(5S)-3-(3,6-dihydro-2H-pyran-4-yl)-7-[5-(prop-1-yn-1-yl)pyridin-3-yl]-5'H-spiro[1-benzopyrano[2,3-c]pyridine-5,4'-[1,3]oxazol]-2'-amine 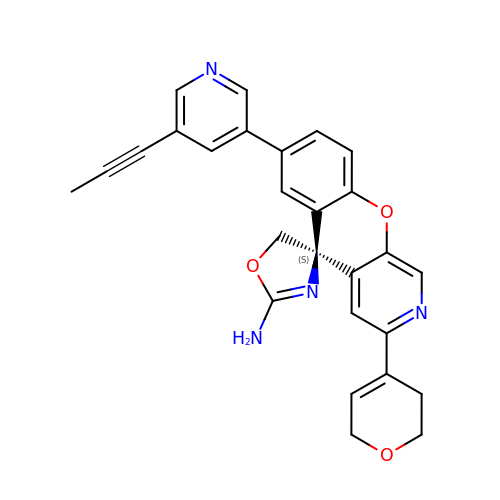| C27 H22 N4 O3 | PAMPHNBKOPBUKU-MHZLTWQESA-N(3R,4S)-1-[(4-amino-5H-pyrrolo[3,2-d]pyrimidin-7-yl)methyl]-4-({[3-(1-benzyl-1H-1,2,3-triazol-4-yl)propyl]sulfanyl}methyl)pyrrolidin-3-ol 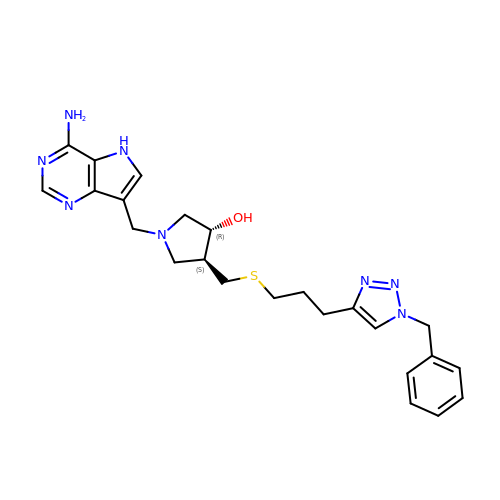| C24 H30 N8 O S | BROXRHKDLDDNBO-CTNGQTDRSA-N> YSLFPNSPKWTSKVVTYRIVSYTRDLPHITVDRLVSKALNMWGKEIPLHFRKVVWGTADIMIGFARGAHGDSYPFDGPGNTLAHAFAPGTGLGGDAHFDEDERWT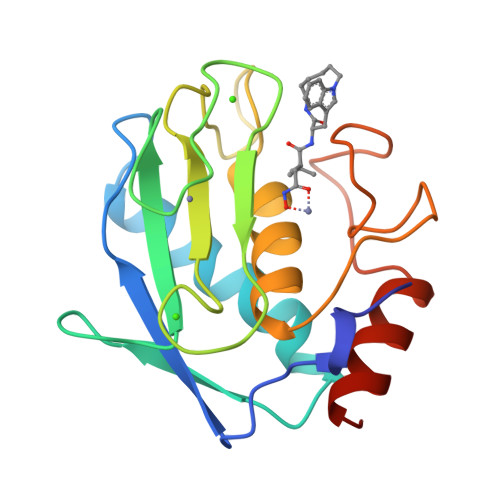DGSSLGINFLYAATHELGHSLGMGHSSDPNAVMYPTYGNGDPQNFKLSQDDIKGIQKLYGKRSNS>[2x]TRDQNGTWEMESNENFEGYMKALDIDFCTRKIAVRLTQ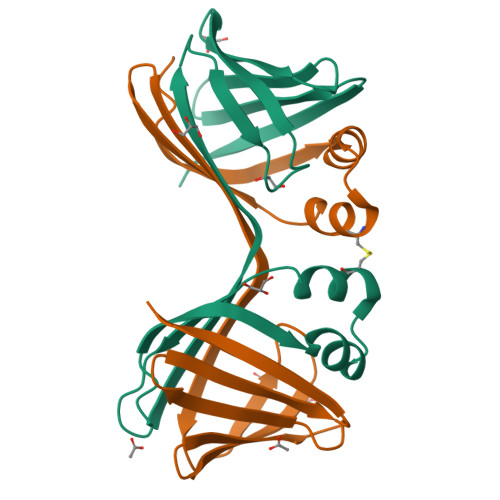TKVIDQDGDNFKDKTTSTFRNYDVDFTVGVEFDEYTKSLDNRHVKALVTWEGDVLVCVQKGEKENRGWKKWIEGDKLYLELTCGDQVCRQVFKKK>SSNDNIELVDFQNIMFYGDAEVGDNQQPFTFILDTGSANLWVPSVKCTTAGCLTKHLYDSSKSRTYEKDGTKVEMNYVSGTVSGFFSKDL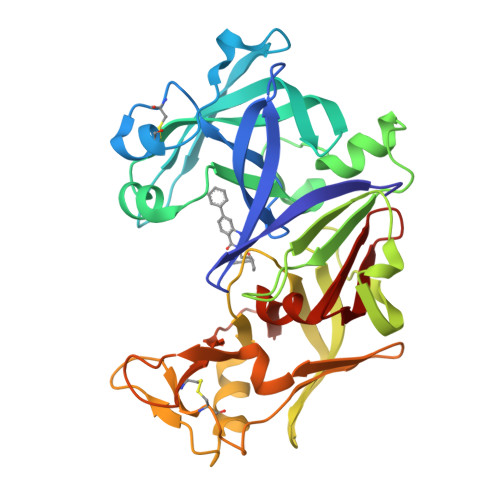VTVGNLSLPYKFIEVIDTNGFEPTYTASTFDGILGLGWKDLSIGSVDPIVVELKNQNKIENALFTFYLPVHDKHTGFLTIGGIEERFYEGPLTYEKLNHDLYWQITLDAHVGNISLEKANCIVDSGTSAITVPTDFLNKMLQNLDVIKVPFLPFYVTLCNNSKLPTFEFTSENGKYTLEPEYYLQHIEDVGPGLCMLNIIGLDFPVPTFILGDPFMRKYFTVFDYDNHSVGIALAKKNL[2x]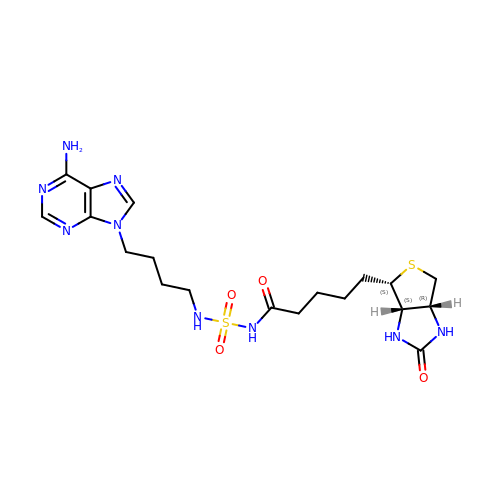N-{[4-(6-amino-9H-purin-9-yl)butyl]sulfamoyl}-5-[(3aS,4S,6aR)-2-oxohexahydro-1H-thieno[3,4-d]imidazol-4-yl]pentanamide | C19 H29 N9 O4 S2 | WPCYKZJXLXIRGW-YDHLFZDLSA-N>GADGNEDLRADDLPGPAFESYESMELACPAERSGHVAVSDGRHMFVWGGYKSNQVRGLYDFYLPREELWIYNMETGRWKKINTEGDVPPSMSGSCAVCVDRVLYLFGGHHSRGNTNKFYMLDSRSTDRVLQWERIDCQGIPPSSKDKLGVWVYKNKLIFFGGYGYLPEDKVLGTFEFDETSFWNSSHPRGWNDHVHILDTETFTWSQPITTGKAPSPRAAHACATVGNRGFVFGGRYRDARMNDLHYLNLDTWEWNELIPQGICPVGRSWHSLTPVSSDHLFLFGGFTTDKQPLSDAWTYCISKNEWIQFNHPYTEKPRLWHTACASDEGEVIVFGGCANNLLVHHRAAHSNEILIFSVQPK[2x];>HSVNQRFGSNNTS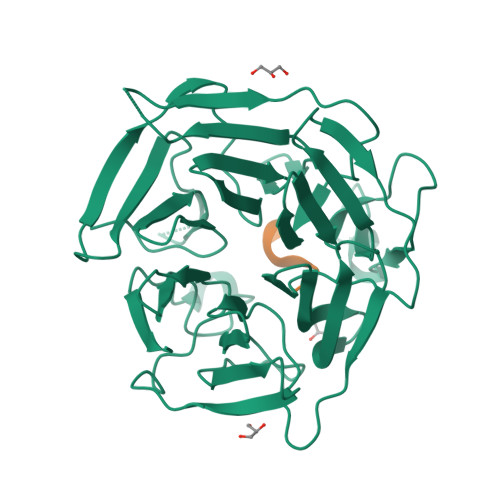GS[2x]>[2x]AKRQWALEDFEIGRPLGKG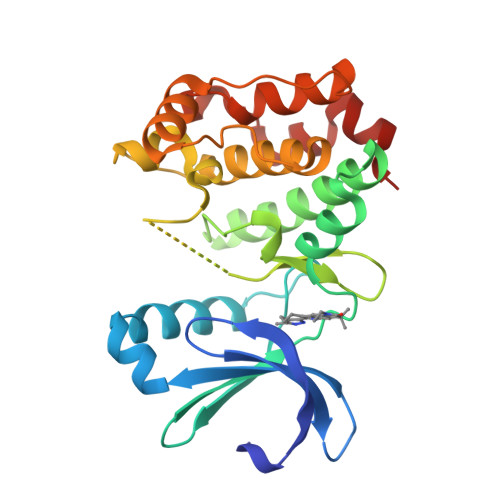KFGNVYLAREKNSKFILALKVLFKAQLEKAGVEHQLRREVEIQSHLRHPNILRLYGYFHDSTRVYLILEYAPLGTVYRELQKLSKFDEQRTATYITELANALSYCHSKKVIHRDIKPENLLLGSAGELKIADFGWSVHAPSSRRAALCGTLDYLPPEMIEGRMHDEKVDLWSLGVLCYEFLVGKPPFEANTYQDTYKRISRVEFTFPDFVTEGARDLISRLLKHNPSQRPMLREVLEHPWITANSSKPS> SLFKDDIQLNEHQVAWYSKDWTAVQSAADSFKEKAENEFFEIIGAINNKTKCSIAQKDYSKFMVENALSQFPECMPAVYAMNLIGSGLSDEAHFNYLMAAVPRGKRYGKWAKLVEDSTEVLIIKLLAKRYQVNTNDAINYKSILTKNGKLPLVLKELKGLVTDDFLKEVTKNVKEQKQLKKLALEWGLEHHHHHHHHHH;>GPGGSMITVNEKEHILEQKYRPSTIDECILPAFDKETFKSITSKGKIPHIILHSPSPGTGKTTVAKALCHDVNADMMFVNGSDCKIDFVRGPLTNFASAASFDGRQKVIVIDEFDRSGLAESQRHLRSFMEAYSSNCSIIITANNIDGIIKPLQSRCRVITFGQPTDEDKIEMMKQMIRRLTEICKHEGIAIADMKVVAALVKKNFPDFRKTIGELDSYSSKGVLDAGILSLVTNDRGAIDDVLESLKNKDVKQLRALAPKYAADYSWFVGKLAEEIYSRVTPQSIIRMYEIVGENNQYHGIAANTELHLAYLFIQLACEMQWK[4x];>[3x]MKLSKDTTALLKNFATINSGIMLKSGQFIMTRAVNGTTYAEANISDVIDFDVAIYDL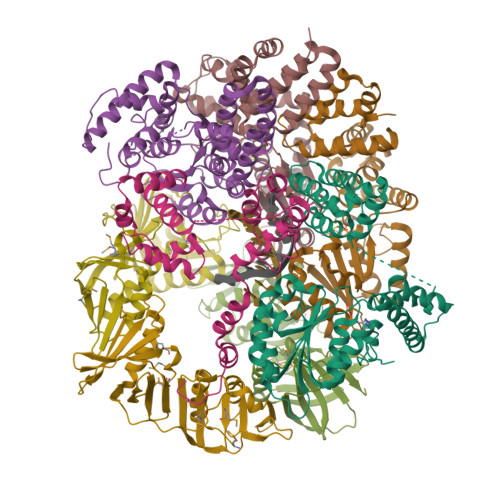NGFLGILSLVNDDAEISQSEDGNIKIADARSTIFWPAADPSTVVAPNKPIPFPVASAVTEIKAEDLQQLLRVSRGLQIDTIAITVKEGKIVINGFNKVEDSALTRVKYSLTLGDYDGENTFNFIINMANMKMQPGNYKLLLWAKGKQGAAKFEGEHANYVVALEADSTHDF>[2x]QRCGSQGGGGTCPALWCCSIWGWCG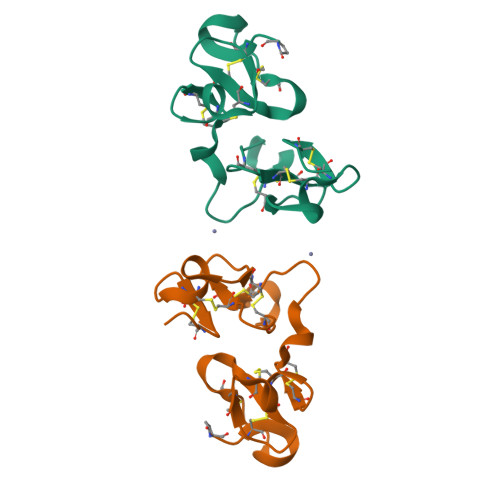DSEPYCGRTCENKCWSGERSDHRCGAAVGNPPCGQDRCCSVHGWCGGGNDYCSGSKCQYRCSSS octyl beta-D-galactopyranoside | C14 H28 O6 | 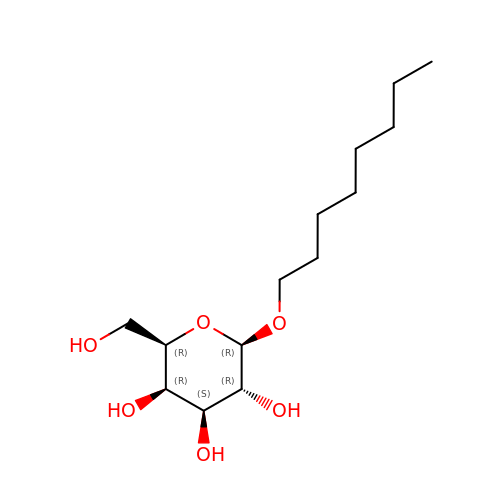HEGSGKPQLMEBJL-MBJXGIAVSA-N>SVKTGIYQVLNGSRLCIKAEMGIQLIVQDKESVFSPRRYFNIDPNATQASGNCGTRKSNLLLNFQGGFVNLTFTKDEESYYISEVGAYLTVSDPETVYQGIKHAVVMFQTAVGHSFKCVSEQSLQLSAHLQVKTTDVQLQAFDFEDDHFGNVDECSSDYTHHHHHH[2x]

The family of lysosome-associated membrane proteins (LAMP) comprises the multifunctional, ubiquitous LAMP-1 and LAMP-2, and the cell type-specific proteins DC-LAMP (LAMP-3), BAD-LAMP (UNC-46, C20orf103) and macrosialin (CD68). LAMPs have been implicated in a multitude of cellular processes, including phagocytosis, autophagy, lipid transport and aging. The five human members of the LAMP protein family are characterized by a conserved 'LAMP domain' directly adjacent to the single transmembrane helix. DC-LAMP is a highly specific marker for mature DCs in humans and other mammals including cattle and pigs, but it is not expressed in DCs of mice.

The crystal structure of the membrane-proximal domain of human DC-LAMP was solved by multi-wavelength anomalous dispersion (MAD) phasing and refined at a resolution of 2.8 Å. Two protein molecules denoted chain A and B are present in the asymmetric unit, which are related to each other by a two-fold non-crystallographic symmetry. Analysis with the protein interfaces, surfaces and assemblies service PISA predicted that the domain is a monomer in solution, in correspondence with gel filtration results. The DC-LAMP domain consists of two β-sheets that form a "pseudo β-prism". The front β-sheet is bent in the middle by two connected β-bulges, which are formed by the β-strand pairs S2/S10 and S10/S9. This bending forms the domain's triangular prism shape and it opens a hydrophobic pocket between the sheets, constituting a possible binding site for small molecules. The conformation of loop L1 and the adjacent β-hairpin formed by strands S7 and S8 differs between chains A and B, due to crystal contacts, indicating that these regions are flexible in solution. Two disulfide bonds and an N-acetylglucosamine residue connected to Asn291 were visible in the DC-LAMP domain's electron density map. The first disulfide bond stabilizes the β-prism by linking its two sheets. The second disulfide bond, linking the front β-sheet and the domain's C-terminus, strengthens the connection of the C-terminal transmembrane helix to the center of the front β-sheet.>[4x]PSETPQAEVGPTGCPHRSGPHSAKGSLEKGSPEDKEAKEPLWIRPDAPSRCTWQLGRPASESPHHHTAPAKSPKILPDILKKIGDTPMVRINKIGKKFGLKCELLAKCEFFNAGGSVKDRISLRMIEDAERDGTLKPGDTIIEPTSGNTGIGLALAAAVRGYRCIIVMPEKMSSEKVDVLRALGAEIVRTPTNARFDSPESHVGVAWRLKNEIPNSHILDQYRNASNPLAHYDTTADEILQQCDGKLDMLVASVGTGGTITGIARKLKEKCPGCRIIGVDPEGSILAEPEELNQTEQTTYEVEGIGYDFIPTVLDRTVVDKWFKSNDEEAFTFARMLIAQEGLLCGGSAGSTVAVAVKAAQELQEGQRCVVILPDSVRNYMTKFLSDRWMLQKGFLKEEDLTEKKPWWWHLRVQELGLSAPLTVLPTITCGHTIEILREKGFNQAPVVDEAGVILGMVTLGNMLSSLLAGKVQP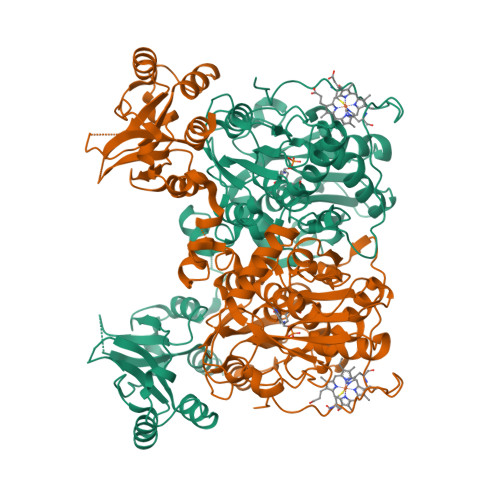SDQVGKVIYKQFKQIRLTDTLGRLSHILEMDHFALVVHEQQRQMVFGVVTAIDLLNFVAAQERDQKLEHHHHHH>[5x]MSNFKVRDPVIQERLDHDYAHHPLVARMNTLDQGNMSQAEYLVQKRHYLVFLIAHHYYEAYLRRMGGIQRRDHLQTLRDQKPRERADRVSAASAYDAGTFTVPSRPGPASGTTPGGQDSLGVSGSSITTLSSGPHSLSPASDILTTLSSTTETAAPAVADARKPPSGKKK;>MEATLEQRPFPYLATEANLLTQIKESAADGLFKSFQLLLGKDAREGSVRFEALLGVYTNVVEFVKFLETALAAACVNTEFKDLRRMIDGKIQFKISMPTIAH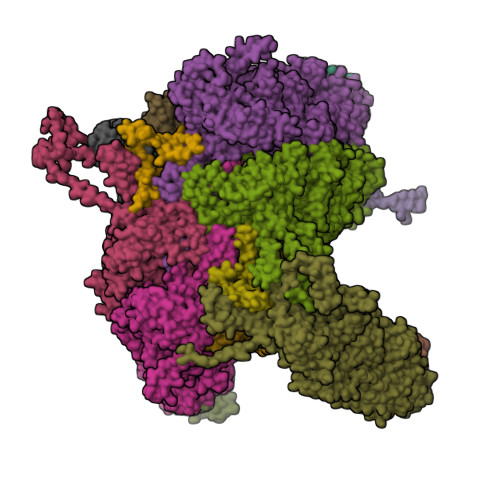GDGRRPNKQRQYIVMKACNKHHIGAEIELAAADIELLFAEKETPLDFTEYAGAIKTITSALQFGMDALERGLVDTVLAVKLRHAPPVFILKTLGDPVYSERGLKKAVKSDMVSMFKAHLIEHSFFLDKAELMTRGKQYVLTMLSDMLAAVCEDTVFKGVSTYTTASGQQVAGVLETTDSVMRRLMNLLGQVESAMSGPAAYASYVVRGANLVTAVSYGRAMRNFEQFMARIVDHPNALPSVEGDKAALADGHDEIQRTRIAASLVKIGDKFVAIESLQRMYNETQFPCPLNRRIQYTYFFPVGLHLPVPRYSTSVSVRGVESPAIQSTETWVVNKNNVPLCFGYQNALKSICHPRMHNPTQSAQALNQAFPDPDGGHGYGLRYEQTPNMNLFRTFHQYYMGKNVAFVPDVAQKALVTTEDLLHPTSHRLLRLEVHPFFDFFVHPCPGARGSYRATHRTMVGNIPQPLAPREFQESRGAQFDAVTNMTHVIDQLTIDVIQETAFDPAYPLFCYVIEAMIHGQEEKFVMNMPLIALVIQTYWVNSGKLAFVNSYHMVRFICTHMGNGSIPKEAHGHYRKILGELIALEQALLKLAGHETVGRTPITHLVSALLDPHLLPPFAYHDVFTDLMQKSSRQPIIKIGDQNYDNPQNRATFINLRGRMEDLVNNLVNIYQTRVNEDHDERHVLDVAPLDENDYNPVLEKLFYYVLMPVCSNGHMCGMGVDYQNVALTLTYNGPVFADVVNAQDDILLHLENGTLKDILQAGDIRPTVDMIRVLCTSFLTCPFVTQAARVITKRDPAQSFATHEYGKDVAQTVLVNGFGAFAVADRSREAAETMFYPVPFNKLYADPLVAATLHPLLANYVTRLPNQRNAVVFNVPSNLMAEYEEWHKSPVAAYAASCQATPGAISAMVSMHQKLSAPSFICQAKHRMHPGFAMTVVRTDEVLAEHILYCSRASTSMFVGLPSVVRREVRSDAVTFEITHEIASLHTALGYSSVIAPAHVAAITTDMGVHCQDLFMIFPGDAYQDRQLHDYIKMKAGVQTGPPGNRMDHVGYAAGVPRCENLPGLSHGQLATCEIIPTPVTSDVAYFQTPSNPRGRAACVVSCDAYSNESAERLLYDHSIPDPAYECRSTNNPWASQRGSLGDVLYNITFRQTALPGMYSPCRQFFHKEDIMRYNRGLYTLVNEYSARLAGAPATSTTDLQYVVVNGTDVFLDQPCHMLQEAYPTLAASHRVMLDEYMSNKQTHAPVHMGQYLIEEVAPMKRLLKLGNKVVY[5x];>[2x]MKVQAENAARLGRQVLGLLPPPTHRVSLTRGPEFARGVRDLLSKYAASTRPTVGSLHEALRQAPFRQPTYGDFLVYSQTFSPQEPLGTFLFSFKQEDNGSSMDMLLTPTSLFMLSGMEAAKAPQTHKVAGVWYGSGSGLADFIPNLSELMDTGEFHTLLTPVGPMVQSVHSTFVTKVTSAMKGVGLARDEPRAHVGLTLPCDMLVDLDESCPMVQRREPAGLNVTIYASLVYLRVNQRPSMALTFFQSGKGFAEVVAMIKDHFTDVIRTKYIQLRHELYINRLVFGAVCTLGTVPFDSHPVHQSLNVKGTSLPVLVFANFEAACGPWTVFL;>[4x]MALDKSIVVNLTSRLFADELAALQSKIGSVLPLGDCHRLQNIQALGLGCVCSRETSPDYIQIMQYLSKCTLAVLEEVRPDSLRLTRMDPSDNLQIKNVYAPFFQWDSNTQLAVLPPLFSRKDSTIVLESNGFDIVFPMVVPQQLGHAILQQLLVYHIYSKISAGAPGDVNMAELDLYTTNVSFMGRTYRLDVDNTDPRTALRVLDDLSMYLCILSALVPRGCLRLLTALVRHDRHPLTEVFEGVVPDEVTRIDLDQLSVPDDITRMRVMFSYLQSLSSIFNLGPRLHVYAYSAETLAASCWYSPR>[3x]SNAMDERFNAALHESAHTVIAQVLGFNTATPIIYENSSTNPDEKHWLGKAFIDTTNGNVEDIALVGLAGEAIQYYIEGVDVGDCPFIWECNLEDISLS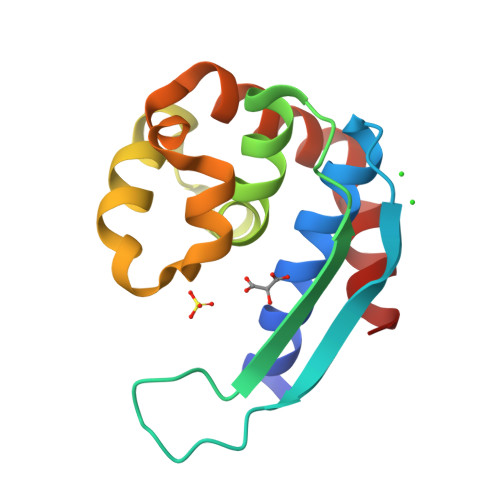DQELVKDLYNDVELWEKLYTLFEQHHDSILDLANSI>GAMGGPEDTTQDDDMKQSIVKWLFELNAKQREVLARRFGLLGYEAATLEDVGREIGLTRERVRQIQVEGLRRLREILQGQGLNIEALFREGSGSKGETQLTPEEKLLRAIFGEKA[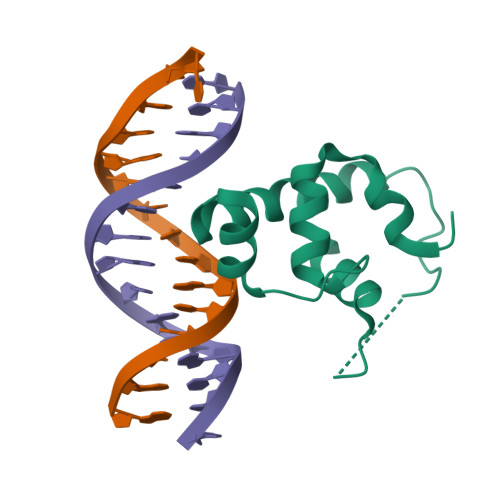2x]> MVRIHLVTWENRKLYRKVLERYFRIRYDIYVKQRRWRAVARPINIEIDAFDNEHALYVLALDANGKIVGGSRLVPTLEPHLMSEVFPILAGGTPPRAAEIFEWTRFFVMPSFRTKGASSPVAGFVLCGLLETAQSLGIRQISVVCETFWPKRLRA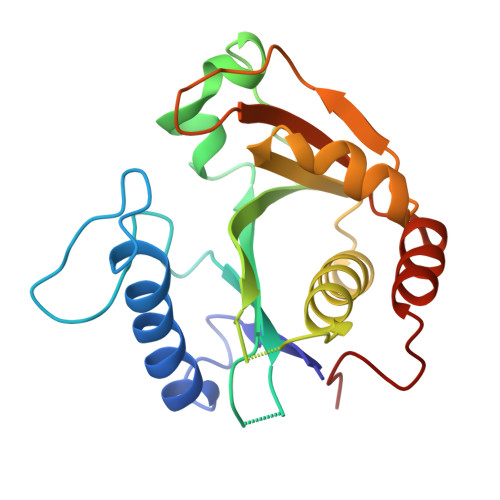LGWTLFELGNALEHPDGDIIALLIDVTPEAIEQTRRAYGISGAILADGI>MGSSHHHHHHHHGASENLYFQGASMTRATNFTELYAGKGILETYMIAEKITRYFTRDLIELSGLLESELSPLKLLDLACGTGVVSERLHEMLASKAPASWELICGDISAELTGHVKRKIIEEGWTNSSARVMDAQNTELATAELTHVFAALAWTSFPDTYAALKDSLRILRPGGTLTISTWQKTEWLGVLEAAVKTIPTRLPFPTTKEFMSCMNPGWDDENYVRGRLEEAGFVHVYSTTISKEFQISTADLYKIAAPVIPIIVSKWWTTEQKEAHEHEILPALAKHLEATYGETG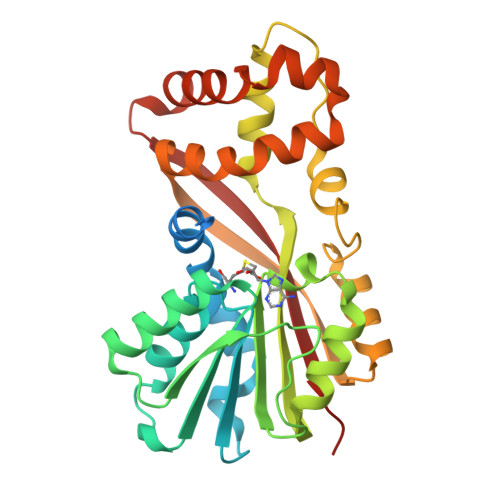LVPQKWTAVFAKGEKEK[2x]PGNs are normally recognized, and/or hydrolyzed (amidases EC 3.5.1.28) in some cases, by a class of PRRs, termed peptidoglycan recognition proteins (PGRPs). The catalytic PGRPs possess the amidase activity that hydrolyzes the amide bond between the MurNAc and L-alanine moieties of PGN, via a coordinated Zn2+ ion. The full-length BbtPGRP3 consists of an N-terminal signal peptide (Met1−Ala18), followed by a CBD (Gln19−Tyr71) and a C-terminal PGRP domain (Thr90−Gly255), which are connected via an 18-residue linker from residues Ser72 to Gly89. All together, the modular evolution via gene horizontal transfer and domain shuffling results in a unique domain organization of BbtPGRP3, which has a higher amidase activity and a broader spectrum against invading bacteria.

Here we report the crystal structure of BbtPGRP3 at 2.7 Å resolution, showing an N-terminal hevein-like CBD followed by a classic PGRP domain at the C-terminus. Each asymmetric unit of the crystal contains one molecule of BbtPGRP3 (covering residues Gln19−Gly74 and Ser87−Gly254). It is composed of an N-terminal CBD (Gln19−Tyr71) and a C-terminal PGRP domain (Thr90−Val254) connected by a truncated linker (Ser72−Gly74, Ser87−Gly89). Notably, truncation of the linker from 18 to 6 residues did not lead to significant change of the amidase activity; thus only the wild-type BbtPGRP3 was applied to all following activity assays and comparisons. The CBD starts with a long N-terminal loop (Gln19−Glu40), followed by the core structure of a three-stranded antiparallel β-sheet (β1~3) and a helix α1. The CBD of BbtPGRP3 adopts an overall structure remarkably similar to the well-characterized U. dioica UDA. Besides, the four disulfide bridges (Cys27-Cys50, Cys41-Cys56, Cys49-Cys63, and Cys65-Cys68) that stabilize the BbtPGRP3 CBD also resemble the counterparts in UDA. All the four putative chitin-binding residues of the CBD of BbtPGRP3 could be superimposed to those in the structure of UDA complexed with a trisaccharide. At the center of the solvent-exposed valley, a zinc ion is tetrahedrally coordinated by the nitrogen atoms of residues His121, His230, the sulfur atom of Cys238, and a water molecule Wat1. Wat1 is further stabilized by the Oη atoms of the catalytic residue Tyr156, which have been proposed to facilitate a water-mediated nucleophilic attack on the lactyl-amide bond and stabilize the reaction intermediate, respectively.

> GSQRWRSDGRCGPNYPAPDANPGECNPHAVDHCCSEWGWCGRETSHCTCSSCVDYSAGSSGTCPRIVSKSEWGSRATNYNVFLSLPVPKVVIHHSAGATCSTQSSCSLQVRNIQNYHMDGRGYSDIGYNFLVGNDGNVYEGRGWDRRGAHALNVNTESIGICFMGDFTSQKPTASAIAAAKSLISCGVSLGKIRSGYSLYGHRDVGSTACPGNLLYDDIKSWGRYVGAAAHHHHHH>[2x]MDLRDIDLNLLVVFNQLLLDRSVSTAGEKLGLTQPAVSNSLKRLRTALNDDLFLRTSKGMEPTPYALHLAEPVIYALNTLQTALTTRDSFDPFASTRTFNLAMTDIGEMYLMPPLMEALAQRAPHIQISTLRPNAGNLKEDMESGAVDLALGLLPELQTGFFQ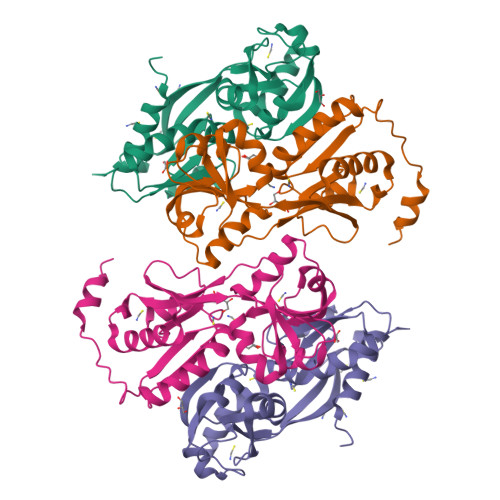RRLFRHRYVCMFRKDHPSAKSPMSLKQFSELEHVGVVALNTGHGEVDGLLERAGIKRRMRLVVPHFIAIGPILHSTDLIATVPQRFAVRCEVPFGLTTSPHPAKLPDIAINLFWHAKYNRDPGNMWLRQLFVELFSEAHHHHHH> SPQPLEQIKLSESQLSGRVGMIEMDLASGRTLTAWRADERFPMMSTFKVVLCGAVLARVDAGDEQLERKIHYRQQDLVDYSPVSEKHLADGMTVGELCAAAITMSDNSAANLLLATVGGPAGLTAFLRQIGDNVTRLDRWETELNEALPGDARDTTTPASMAATLRKLLTSQRLSARSQRQLLQWMVDDR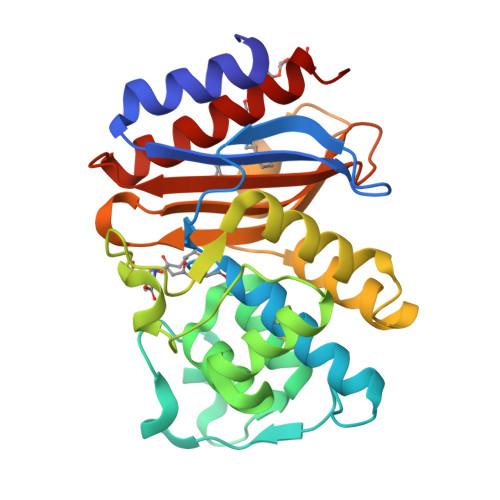VAGPLIRSVLPAGWFIADRTGAGERGARGIVALLGPNNKAERIVVIYLRDTPASMAERNQQIAGIGAALIEHWQR Terminal uridylyl transferase (TUTase) is one type of enzyme that modifies RNA molecules by facilitating the post-transcriptional addition of uridyl ribonucleotides to their 3′ ends. Recent researches have reported that Drosophila TUTase, Tailor, exhibits an intrinsic preference for RNA substrates ending in 3′G, distinguishing it from any other known TUTases. Through this unique feature, Tailor plays a crucial role as the repressor in the biogenesis pathway of splicing-derived mirtron pre-miRNAs. The structure of Tailor contains two canonical globular domains separated by a large catalytic groove, which serves to accommodate the 3′ ends of the target RNAs for the post-transcriptional addition of uridyl ribonucleotides.

Three complex structures of Tailor-AGU, Tailor-AGUU and Tailor-U4 (Tailor-UUUU) we obtained in this research were respectively designed to mimic the post-catalytic states of the addition of the first and second uridines as well as the extension of polyuridylation chain. As indicated by the structural analysis, the terminal Us in both Tailor-AGU and Tailor-AGUU adopt a very similar conformation at the +1 position (U+1) as their equivalent nucleotides in previously reported structures, interacting with the surrounding residues through extensive direct and water-mediated hydrogen bonds, as well as hydrophobic interactions. More specifically, the O2 carbonyl group and 2′-hydroxyl group of U+1 make two direct hydrogen bonds with the side-chain group of N353. Furthermore, the side-chain of T354 contributes to the generation of water-mediated hydrogen bonds with 2′- and 3′-hydroxyl groups of U+1, while U+1 base forms hydrophobic stacking interaction against the aromatic side-chain of Y390 and an additional hydrophobic interaction with the main chain of V542, as well as a water-mediated hydrogen-bonding network with D515, Q519, and H522 from NRM loop. At the 0 nucleotide-binding position which is occupied by a guanine (G0) and a uridine (U0) in two complexes, respectively, protein-RNA recognition modes are similar but not identical. In Tailor-AGU, the O6 carbonyl group and N7 imino proton of G0 form totally three hydrogen bonds with the guanidine groups of R327 from the loop connecting β3 and β4 strands while the NH2 group of G0 is involved in a hydrogen bond with the side-chain group of N347, ensuring this guanine is specifically recognized by Tailor. Other than these direct recognitions, G0 base also makes water-mediated hydrogen bonding interactions with the side-chain groups of N347 and Q519, and a hydrophobic interaction with the side-chain group of V328. 5′A at the -1 position (A-1) in Tailor-AGU is less restricted by the interactions with the protein except the hydrophobic interactions with I323 and I330 and a water-mediated hydrogen bond between 2′-hydroxyl group and main chain atom of V328. R327 and N347 are key residues in forming direct hydrogen bonds with G0.

> HMQHITVRLPKKARAMIVGEITNVFKDKYPIADKLKVIPEYDVIEQDLCKLLSPGFPKQPLRVYKFGSRITGIGNRSSDLDLFVDIGNTFHTFEHRASNATVAKLRAMRKFFCDSEDWRLINFIEQARVPIIKTCHLPTGIECDICLNSMGFCNTNLLKYIFESQPLTQYMCIYVKNWLERCKLTEQISTYSITLMVIYFLQLQALLPPIAMLQIEDAANQAVLVGPWVVNFAQKSFSELGLQQLKATVPVIKGFLRNFFAYFAKFDYEHFLVCPYIGQANVEIAKIERMLHARYSAYVSDNPECSIQLKKPMVVQDPIQLNHNVTKAVTKYGLQTFVDYCQQTAELLEEP>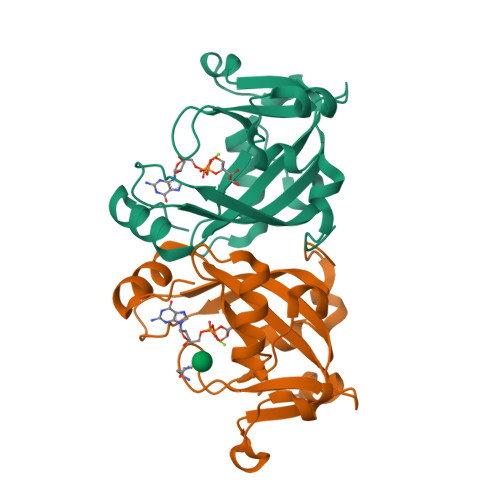MMFLRQEDFATVVRSTPLVSLDFIVENSRGEFLLGKRTNRPAQGYWFVPGGRVQKDETLEAAFERLTMAELGLRLPITAGQFYGVWQHFYDDNFSGTDFTTHFVVLGFRFRVSEEELLLPDEQHDDYRWLTSDALLASDNVHANSRAYFLAEKRTGVPGL[3x]> KENA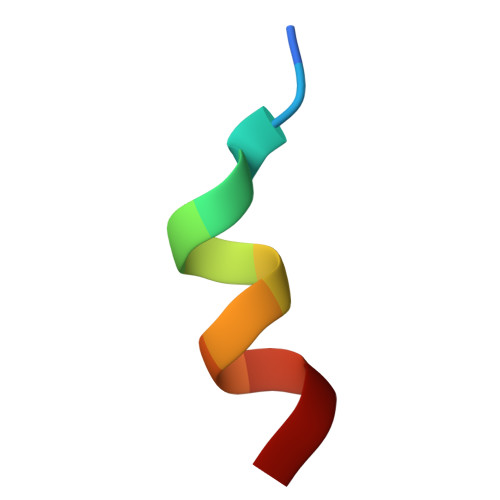LLRYLLDK>[2x]GSHMGGERTVTIRRQTVGGFGLSIKGGAEHNIPVVVSKISKEQRAELSGLLFIGDAILQINGINVRKCRHEEVVQVLRNAG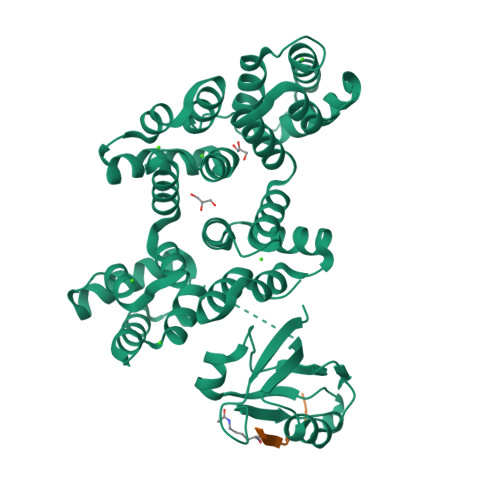EEVTLTVSFLKRAPGSAYGSVKAYTNFDAERDALNIETAIKTKGVDEVTIVNILTNRSNEQRQDIAFAYQRRTKKELASALKSALSGHLETVILGLLKTPAQYDASELKASMKGLGTDEDSLIEIICSRTNQELQEINRVYKEMYKTDLEKDIISDTSGDFRKLMVALAKGRRAEDGSVIDYELIDQDARDLYDAGVKRKGTDVPKWISIMTERSVPHLQKVFDRYKSYSPYDMLESIRKEVKGDLENAFLNLVQCIQNKPLYFADRLYDSMKGKGTRDKVLIRIMVSRSEVDMLKIRSEFKRKYGKSLYYYIQQDTKGDYQKALLYLCGGDD;>[2x]EDQHTQITKV>SIDQSVVISEKFANSIFAAVEHIKKQIKERDSNYKAIIFAPTVKFTSFLCSILKNEFKKDLPILEFHGKITQNKRTSLVK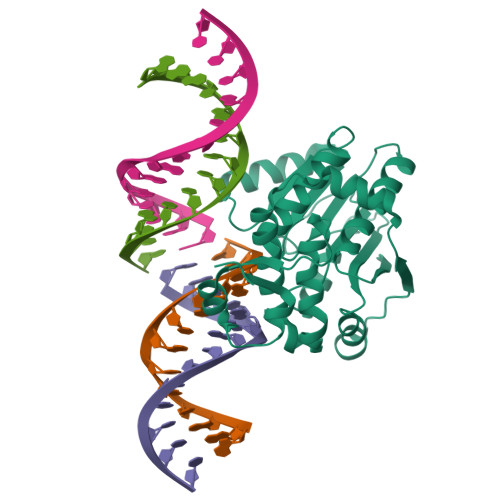RFKKDESGILVCTDVGARGMDFPNVHEVLQIGVPSELANYIHRIGRTARSGKEGSSVLFICKDELPFVRELEDAKNIVIAKQEKYEPSEEIKSEVLEAVTEEPEDISDIVISLISSYRSCIKEYRFSERRILPEIASTYGVLLNDPQLKIPVSRRFLDKLGLSRSPIGKAMFEIRD[2x]>GSHMASALIELKNRILAVLNKLSDRDTQQLAVEELERIAQSLSPEGIALFLTCLYDTDSQQKSVVRRECIRLVGT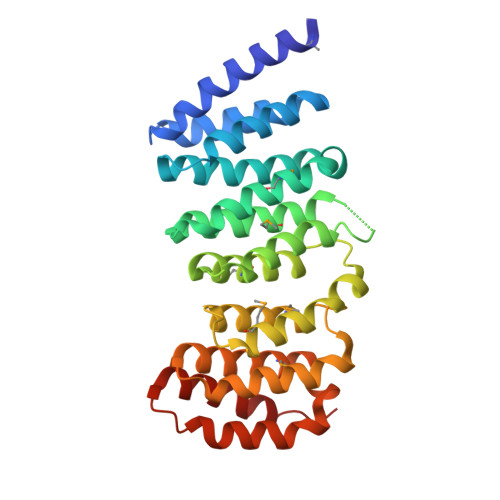LASIHGDLLASHLPKMVANIVKRLKDPDSNIRDACVESMGVLASSIGGADSGAVTTVFVKPLFEALAEQHKTLQTGAAMCLARVLECVKEPHPPTLQRLCPRILKMLASPNFLAKASLLSAVGVMVQVPGVVSASQLPVLLGAVQDELGNSEWAVRKAAAEALSCMASAVGNSLVSYRAGVIAALESSRFDKVKPVRDSVTEALQLWKAIYD[2x]> MRGSHHHHHHGSHVISSIASSLKTAPVIVWFRKDLRLSDNLALLAAVEHGGPVIPVYIREKSAGPLGGAQEWWLHHSLAALSSSLEKAGGRLVLASGDAERILRDLISETGADTVVWNRRYDPTGMATDKALKQKLRDDGLTVRSFSGQLLHEPSRLQTKSGGPYRVYTPFWRALEGSDEPHAPADPPKSLTAPKVWPKSEKLSNWKLLPTKPDWAKDFSDIWTPGETGALDKLDDFIDGALKGYEEGRDFPAKPATSLLSPHLAAGEISPAAVWHATKGLSRHIASNDISRFRKEIVWREFCYHLLFHFPELGEKNWNDSFDAFSWRDDEKSFKAWTRGMTGYPIVDAGMRQLWQHGTMHNRVRMIV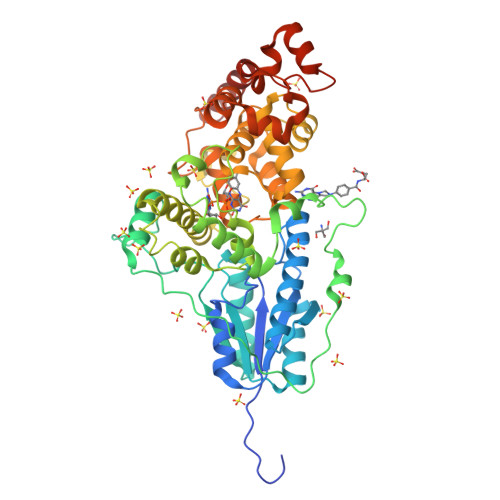ASFLIKHLLIDWRKGEKWFRDTLVDADPASNAANWQWVAGSGADASPFFRIFNPILQGEKFDGDGDYVRRFVPELEKLERKYIHKPFEAPKDALKKAGVELGKTYPLPIVDHGKARERALAAYAAVKKTT>DHNFMRREIKIEGDLVLGGLFPINEKGTGTEECGRINEDRGIQRLEAMLFAIDEINKDNYLLPGVKLGVHILDTCSRDTYALEQSLEFVRASLTKVDEAEYMCPDGSYAIQENIPLLIAGVIGGSYSSVSIQVANLLRLFQIPQISYASTSAKLSDKSRYDYFARTVPPDFYQAKAMAEILRFFNWTYVSTVASEGDYGETGIEAFEQEARLRNICIATAEKVGRSNIRKSYDSVIRELLQKPNARVVVLFMRSDDSRELIAAANRVNASFTWVASDGWGAQESIVKGSEHVAYGAITLELASHPVRQFDRYFQSLNPYNNHRNP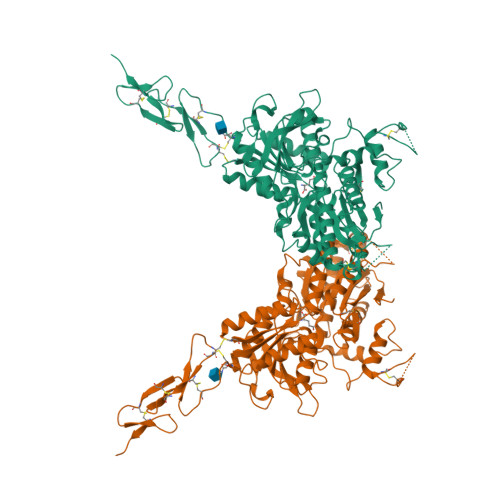WFRDFWEQKFQCSLQNKRNHRQVCDKHLAIDSSNYEQESKIMFVVNAVYAMAHALHKMQRTLCPQTTKLCDAMKILDGKKLYKEYLLKIQFTAPFNPNKGADSIVKFDTFGDGMGRYNVFNLQQTGGKYSYLKVGHWAETLSLDVDSIHWSRNSVPTSQCSDPCAPNEMKNMQPGDVCCWICIPCEPYEYLVDEFTCMDCGPGQWPTADLSGCYNLPEDYIKWEDALVPR[2x]> GLGDLIEGVVEGVTRNALTPLTPANNLPDTQSSGPAHSKETPALTAVETGATNPLVPSDTVQTRHVIQKRTRSESTVESFFARGACVAIIEVDNDAPTKRASKLFSVWKITYKDTVQLRRKLEFFTYSRFDMEFTFVVTSNYTDANNGHALNQVYQIMYIPPGAPIPGKWNDYTWQTSSNPSVFYTYGAPPARISVPYVGIANAYSHFYDGFAKVPLAGQASTEGDSLYGAASLNDFGSLAVRVVNDHNPTKLTSKIRVYMKPKHVRVWCPRPPRAVPYYGPGVDYKDGLAPLPGKGLTTY;> SPNIEACGYSVRVMQLTLGNSTITTQEAANSVVAYGRWPEYIKDSEANPVDQPTEPDVAACRFYTLDTVTWRKESRGWWWKLPDALKDMGLFGQNMFYHYLGRAGYTVHVQCNASKFHQGALGVFAVPEMCLAGDSTTHMFTKYENANPGEKGGEFKGSFTLDTNATNPARNFCPVDYLFGSGVLAGNAFVYPHQIINLRTNNCATLVLPYVNSLSIDSMTKHNNWGIAILPLAPLDFATESSTEIPITLTIAPMCCEFNGLRNITVPRTQ;> GLPVLNTPGSNQYLTADNYQSPCAIPEFDVTPPIDIPGEVRNMMELAEIDTMIPLNLTNQRKNTMDMYRVELNDAAHSDTPILCLSLSPASDPRLAHTMLGEILNYYTHWAGSLKFTFLFC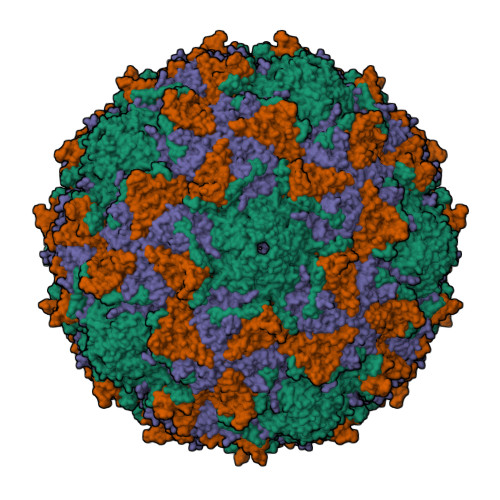GSMMATGKLLVSYAPPGAEAPKSRKEAMLGTHVIWDIGLQSSCTMVVPWISNTTYRQTINDSFTEGGYISMFYQTRVVVPLSTPRKMDILGFVSACNDFSVRLLRDTTHISQEAMPQ;> GAQVSSQKVGAHENSNRAYGGSTINYTTINYYRDSASNAASKQDFAQDPSKFTEPIKDVLIKTAPTLN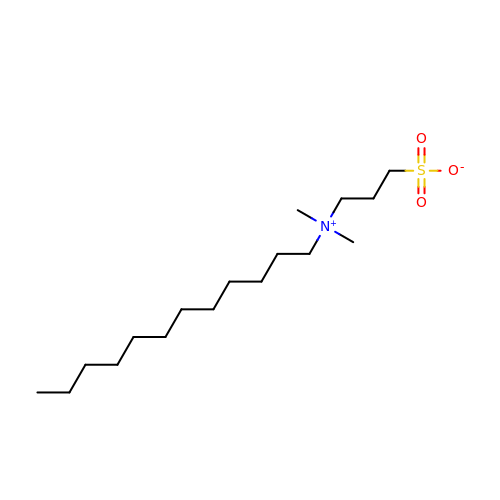3-[DODECYL(DIMETHYL)AMMONIO]PROPANE-1-SULFONATE | C17 H37 N O3 S | IZWSFJTYBVKZNK-UHFFFAOYSA-N>[8x]GSMIELEFHDVAANTSSTFDPEVAYANFKRVHTTGLSYDHIRIFYIKGREIKTSLAKRSEWEVTLNLGGWKITVYNTNFPGNRNNPVPDDGLTLHRLSGFLARYLLEKMLKVSE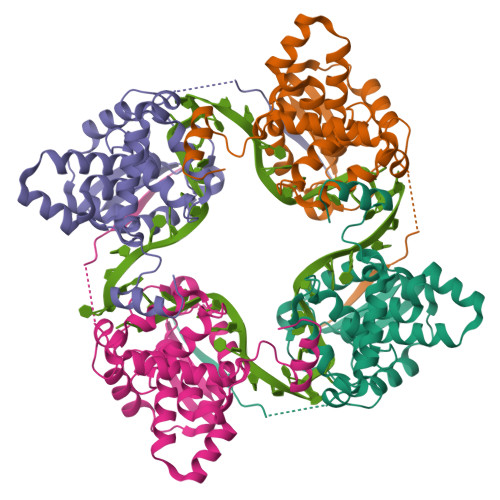PEKLIIKSKIINPLAEKNGITWNDGEEVYLSFFPGSEMFLGTFRFYPLAIGIYKVQRKEMEPKYLEKTMRQRYMGLEAATWTVSKLTEVQSALTVVSSLGWKKTNVSAAARDFLAKFGINM>[6x]MSPKTVFSTDTHREPIPPQPHPSGARPPQLPRELI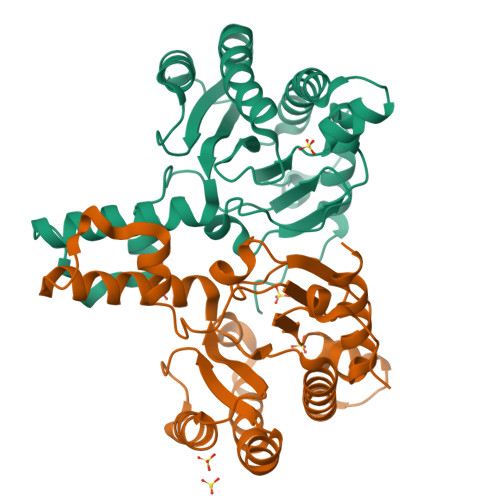PRHVAIVMDGNGRWAKQRGLPRTEGHKAGESSLFDVIEGALELGVPYLSAYAFSTENWKRSPDEVRFLMGFNRDVIRRRRDELHARGVRVRWAGRPGRLWKSVIKELTEAEELTKHNTKLTLQFCVNYGGRAEIADAAAALARDVAAGRLSPNRVTEATLARYLYHPDIPDVDLFIRSSGEQRLSNFLLWQSSYAEFVFLDTLWPDFDRRHFWQACEIYARRDRRYGGAEPNPVGPPQSAAGAQGQD>[2x]GAAEAGITGTWYNQLGSTFIVTAGADGALTGTYESAVGNAESRYV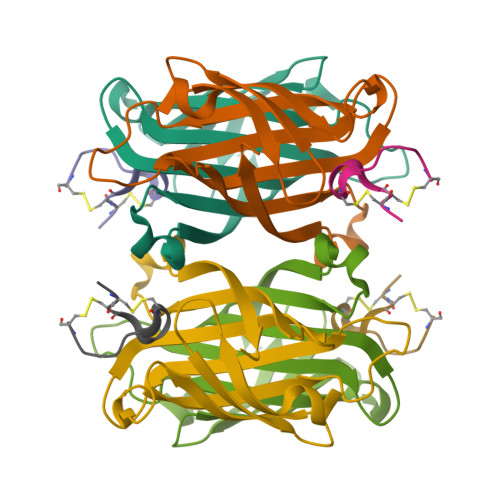LTGRYDSAPATDGSGTALGWTVAWKNNYRNAHSATTWSGQYVGGAEARINTQWLLTSGTTEANAWKSTLVGHDTFTKVKPSAAS;>RCCHPQCGMVEECR[2x]To exert full kinase activity, MST1/2 and LATS1/2 requires coactivators, the scaffolding proteins Salvador homolog 1 (SAV1) and Mps One binder 1 (MOB1), respectively. Phosphorylated MOB1 protein is switched ON to increase the binding affinity to LATS1/2 and this binding accelerates auto-phosphorylation of the activation loop, A-loop (also referred to as activation segment or T-loop), of LATS1/2 kinases for full activation. The phosphorylation of MOB1 occurs at two threonine residues, Thr12 and Thr35, located at the N-terminal extension out of the C-terminal globular MOB core domain, and is required for binding to LATS/NDR kinases. Here we report the results of structural and biochemical studies of full-length mouse MOB1B in the autoinhibited form and that of the MOB core domain bound to the NTR region of LATS1 (hereafter referred to as the MOB1B-LATS1 complex).

We determined the structure of the complex between the N-truncated dominant active form of MOB1B in complex with the NTR domain of LATS1 to independently ascertain which structure of the MOB1-LATS1 complex is correct. The crystal structure of the complex between the NTR (residues 621-703) domain and N-terminal truncated MOB1B (33-216) was determined at 2.96 Å resolution. The structure reveals that the NTR domain forms a V-shaped bihelical structure formed by antiparallel long helices, αA (Gln636-Met668) and αB (Gln674-Ala697), which bind the negatively-charged and nonpolar patched surface of MOB1B. The V shape of the NTR domain is stabilized by formation of an inter-helical hydrophobic core with nonpolar residues (Leu663 and Met667 from the α1 helix, Leu672 from the connected loop, and Met680 and Leu684 from the α2 helix) and inter-helical salt bridges comprising residues, Arg659-Glu688 and Glu664-Arg681. The obtained structure is essentially the same as that of the pMOB1A-LATS1 complex, with small overall root mean square (r.m.s.) deviation (0.79 Å). The helical axis of the αA helix is kinked at His645 with the following part of the αA helix docked into the hydrophobic groove between antiparallel helices H2 and H7, and the αB helix interacts with the negatively-charged patch. Four negatively-charged acidic residues (Glu49 and Glu51 from the H1-H2 loop, and Glu55 and Asp63 from the H2 helix) of MOB1B form direct salt bridge/hydrogen bond formations with six positively-charged residues (His645, Arg656, Arg659 and Lys660 from the α1 helix, and Arg693 and Arg696 from the α2 helix) from the NTR domain. The observed MOB1B-LATS1 interactions in our structure were verified with mutational analysis. Alanine mutants of highly conserved arginine residues (R656A, R693A and R696A) displayed decreased binding affinity to less than 20% of the wild-type.

> GPEATLGSGNLRMAVMLPEGEDLNEWVAVNTVDFFNQINMLYGTITDFCTEESCPVMSAGPKYEYHWADGTNIKKPIKCSAPKYIDYLMTWVQDQLDDETLFPSKIGVPFPKNFMSVAKTILKRLFRVYAHIYHQHFDPVIQLQEEAHLNTSFKHFIFFVQEFNLIDRRELAPLQELIEKLTSKDR;> GPKDEERRESRIQSYSPQAFKFFMEQHVENVLKSHQQRLHRKKQLENEMMRVGLSQDAQDQMRKMLCQKESNYIRLKRAKMDKSM>[4x]MQIKIKYLDETQT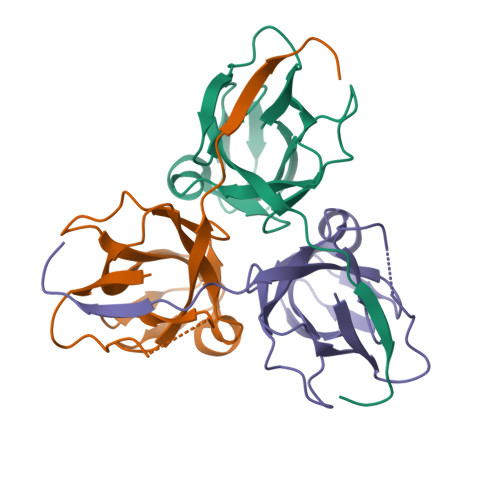RINKMEQGDWIDLRAAEDVAIKKDEFKLVPLGVAMELPEGYEAHVVPRSSTYKNFGVIQTNSMGVIDESYKGDNDFWFFPAYALRDTKIKKGDRICQFRIMKKMPAVDLIEVDRLGNGDRGGHGSTGTK> GSHMTDLPRLPFDNPDIMGIAPQMLALQKEGPIARVGTAGEDAWLVTRYDEVRTLLADRRLRLSNPNPQPSAKSAARAFMVALCAGDDHETEPARHAQMRSLLIPRFSTRRLRLMKTRIEHHVDELLDQLAASAPPVDLHRVLSFRLPTMVVCDLLGVPLADRERFGQWARGTFDQSDNEHSANTFQQVVDYMLELVARKRVEPGDDILSELIAEKDGA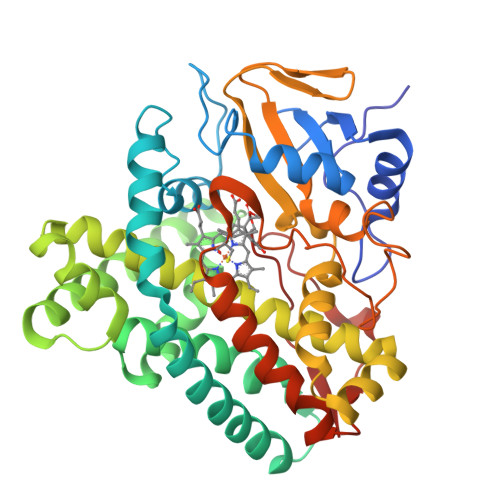LSDADIAHLGNAVLLFGYETTIVRIDLGTLLLLRNPVQRAQLAEDPGLAPAAVEEILRLGVGGKGSNALIPRYAHGDITVGETVIRTGDAVMLAIGAANYDDRAFPDGGLFDLTRVRPRSHLAFGHGARHCIGRTLARIELTAVFERLFRRLPDLRLAVPEESLRWQEHRITGGFDEIPVTF> MSDITKIKQEFDKKVAEIQALMKNPQQDSGLLSNSIDFRDQNLIFSNSGGVCTSSKDKIENYP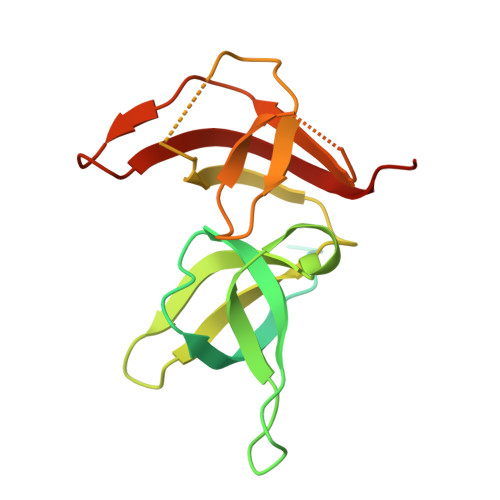AKGYPYKRGVKLSFGDGTTELEVEAGGGDDLYGVCSDIDEFSGMATVIPITNNFTGYLTLKKDGQNGVNPGDKLNFNQHGELEKVTGAQKSVNAIALSKAHKLTEDLFIVLASVFGNRAIKG>[2x]MENTENSVDSKSIKNLEPKIIHGSESMDSGISLDNSYKMDYPEMGLCIIINNKNFHKSTGMTSRSGTDVDAANLRETFRNLKYEVRNKNDLTREEIVELMRDVSKEDHSKRSSFVCVLLSHGEEGIIFGTNGPVDLKKITNFFRGDRCRSLTGKPKLFIIQACRGTELDCGIETD;>SGVDDDMACHKIPVEADFLYAYSTAPGYYSWRNSKDGSWFIQSLCAMLKQYADKLEFMH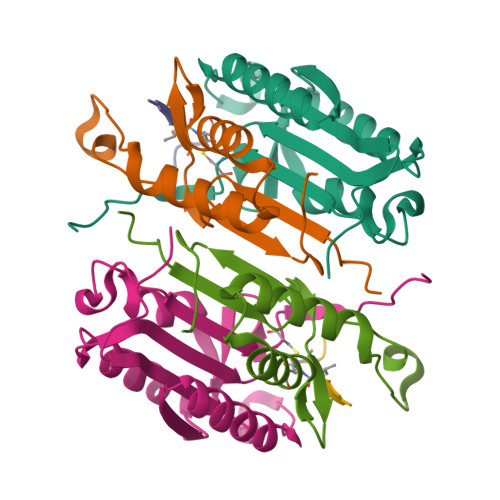ILTRVNRKVATEFESFSFDATFHAKKQIPCIVSMLTKELYFYHLEHHHHHH[2x]>MGSSHHHHHHSQDPMSTGTFVVSQPLNYRGGARVEPADASGTEKAFEPATGRVIATFTCSGEKEVNLAVQNAKAAFKIWSQKSGMERCRILLEAARIIREREDEIATMECINNGKSIFEARLDIDISWQCLEYYAGLAASMAGEHIQLPGGSFGYTRREPLGVCVGIGAWNYPFQIASWKSAPALACGNAMVFKPSPFTPVSALLLAEIYSEAGVPPGLFNVVQGGAATGQFLCQHPDVAKVSFTGSVPTGMKIMEMSAKGIKPVTLELGGKSPLIIFSDCDMNNAVKGALMANFLTQGQVCCNGTRVFVQKEI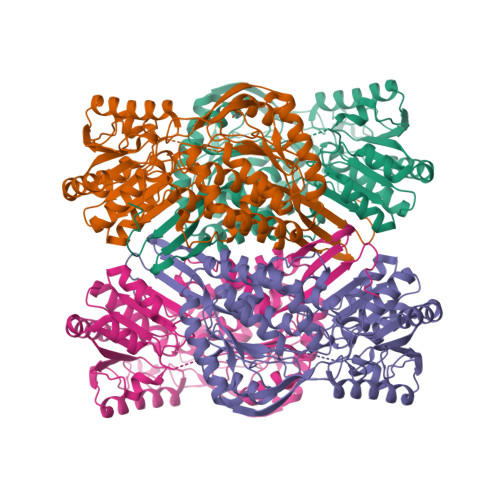LDKFTEEVVKQTQRIKIGDPLLEDTRMGPLINRPHLERVLGFVKVAKEQGAKVLCGGDIYVPEDPKLKDGYYMRPCVLTNCRDDMTCVKEEIFGPVMSILSFDTEAEVLERANDTTFGLAAGVFTRDIQRAHRVVAELQAGTCFINNYNVSPVELPFGGYKKSGFGRENGRVTIEYYSQLKTVCVEMGDVESAF[8x]>SNAMTAVNYPFVDTMDKFDKITKGLIFEHQAEGESETMISHELSILDNDGVVHSLHFSQITSLIDTITGKHPSLELPPQLFLITQYLLEDLKEVGEKGFVITEYFIDVLPTGNKAIFRGTLAHKSTVDGHPDFDPSSTISKKEFEFSLNQFSILQQIALSHCIANLHEECAGF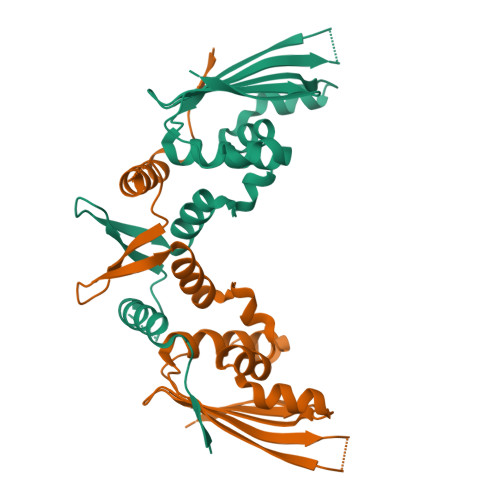RGTFDVEYTFHWTPFAFNVKFSE[4x]>MSSSNVEVFIPVSQGNTNGFPATASNDLKAFTEGAVLSFHNICYRVKLKSGFLPCRKPVEKEILSNINGIMKPGLNAILGPTGGGKSSLLDVLAARKDPSGLSGDVLINGAPRPANFKCNSGYVVQDDVVMGTLTVRENLQFSAALRLATTMTNHEKNERINRVIQELGLDKVADSKVGTQFIRGVSGGERKRTSIGMELITDPSILFLDQPTTGLDSSTANAVLLLLKRMSKQGRTIIFSIHQPRYSIFKLFDSLTLLASGRLMFHGPAQEALGYFESAGYHCEAYNNPADFFLDIINGDSTAVALNREEDFKATEIIEPSKQDKPLIEKLAEIYVNSSFYKETKAELHQLSGGEKKKKITVFKEISYTTSFCHQLRWVSKRSFKNLLGNPQASIAQIIVTVVLGLVIGAIYFGLKNDSTGIQNRAGVLFFLTTNQCFSSVSAVELFVVEKKLFIHEYISGYYRVSSYFLGKLLSDLLPMRMLPSIIFTCIVYFMLGLKPKADAFFVMMFTLMMVAYSASSMALAIAAGQSVVSVATLLMTICFVFMMIFSGLLVN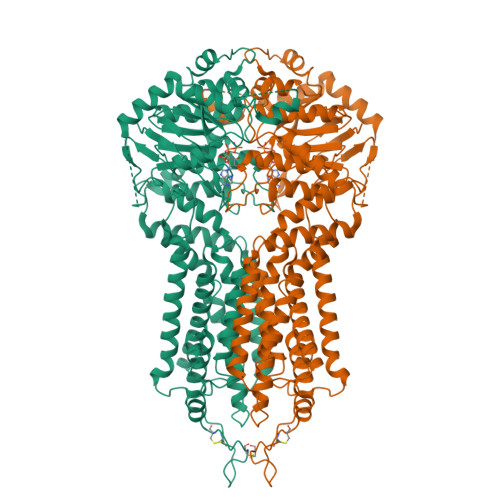LTTIASWLSWLQYFSIPRYGFTALQHNEFLGQNFCPGLNATGNNPCNYATCTGEEYLVKQGIDLSPWGLWKNHVALACMIVIFLTIAYLKLLFLKKYS[2x]> GEIRPTIGQQMETGDQRFGDLVFRQLAPNVWQHTSYLDMPGFGAVASNGLIVRDGGRVLVVDTAWTDDQTAQILNWIKQEINLPVALAVVTHAHQDKMGGMDALHAAGIATYANALSNQLAPQEGMVAAQHSLTFAANGWVEPATAPNFGPLKVFYPGPGHTSDNITVGIDGTDIAFGGCLIKDSKAKSLGNLGDADTEH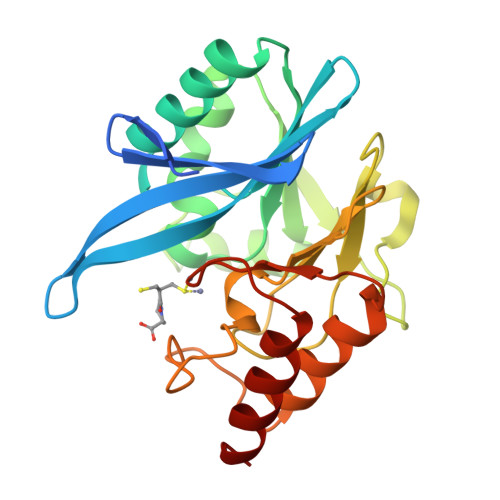YAASARAFGAAFPKASMIVMSHSAPDSRAAITHTARMADKLR(3beta,5beta,9beta)-3-(acetyloxy)cholan-24-oic 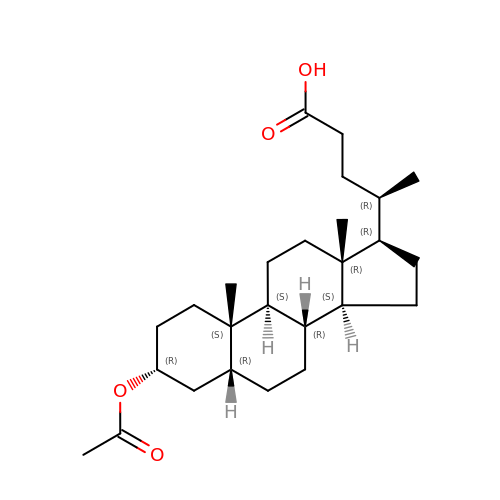acid | C26 H42 O4 | FCQRLHQHKFKTQE-HCTDMSSWSA-N> MVYSYTEKKRIRKDFGKRPQVLDVPYLLSIQLDSFQKFIEQDPEGQYGLEAAFRSVFPIQSYSGNSELQYVSYRLGEPVFDVQECQIRGVTYSAPLRVKLRLVIYEREAPEGTVKDIKEQEVYMGEIPLMTDNGTFVINGTERVIVSQLHRSPGVFFDSDKGKTHSSGKVLYNARIIPYRGSWLDFEFDPKDNLFVRIDRRRKLPATIILRALNYTTEQILDLFFEKVIFEIRDNKLQMELVPERLRGETASFDIEANGKVYVEKGRRITARHIRQLEKDDVKLIEVPVEYIAGKVVAKDYIDESTGELICAANMELSLDLLAKLSQSGHKRIETLFTNDLDHGPYISETLRVDPTNDRLSALVEIYRMMRPGEPPTREAAESLFENLFFSEDRYDLSAVGRMKFNRSLLREEIEGSGILSKDDIIDVMKKLIDIRNGKGEVDDIDHLGNRRIRSVGEMAENQFRVGLVRVERAVKERLSLGDLDTLMPQDMINAKPISAAVKEFFGSSQLSQFMDQNNPLSEITHKRRISALGPGGLTRERAGFEVRDVHPTHYGRVCPIETPEGPNIGLINSLSVYAQTNEYGFLETPYRKVTDGVVTDEIHYLSAIEEGNYVIAQANSNLDEEGHFVEDLVTCRSKGESSLFSRDQVDYMDVSTQQVVSVGASLIPFLEHDDANRALMGANMQRQAVPTLRADKPLVGTGMERAVAVDSGVTAVAKRGGVVQYVDASRIVIKVNEDEMYPGEAGIDIYNLTKYTRSNQNTCINQMPCVSLGEPVERGDVLADGPSTDLGELALGQNMRVAFMPWNGYNFEDSILVSERVVQEDRFTTIHIQELACVSRDTKLGPEEITADIPNVGEAALSKLDESGIVYIGAEVTGGDILVGKVTPKGETQLTPEEKLLRAIFGEKASDVKDSSLRVPNGVSGTVIDVQVFTRDGVEKDKRALEIEEMQLKQAKKDLSEELQILEAGLFSRIRAVLVAGGVEAEKLDKLPRDRWLELGLTDEEKQNQLEQLAEQYDELKHEFEKKLEAKRRKITQGDDLAPGVLKIVKVYLAVKRRIQPGDKMAGRHGNKGVISKINPIEDMPYDENGTPVDIVLNPLGVPSRMNIGQILETHLGMAAKGIGDKINAMLKQQQEVAKLREFIQRAYDLGADVRQKVDLSTFSDEEVMRLAENLRKGMPIATPVFDGAKEAEIKELLKLGDLPTSGQIRLYDGRTGEQFERPVTVGYMYMLKLNHLVDDKMHARSTGSYSLVTQQPLGGKAQFGGQRFGEMEVWALEAYGAAYTLQEMLTVKSDDVNGRTKMYKNIVDGNHQMEPGMPESFNVLLKEIRSLGINIELEDE;> MKDLLKFLKAQTKTEEFDAIKIALASPDMIRSWSFGEVKKPETINYRTFKPERDGLFCARIFGPVKDYECLCGKYKRLKHRGVICEKCGVEVTQTKVRRERMGHIELASPTAHIWFLKSLPSRIGLLLDMPLRDIERVLYFESYVVIEGGMTNLERQQILTEEQYLDALEEFGDEFDAKMGAEAIQALLKSMDLEQECEQLREELNETNSETKRKKLTKRIKLLEAFVQSGNKPEWMILTVLPVLPPDLRPLVPLDGGRFATSDLNDLYRRVINRNNRLKRLLDLAAPDIIVRNEKRMLQEAVDALLDNGRRGRAITGSNKRPLKSLADMIKGKQGRFRQNLLGKRVDYSGRSVITVGPYLRLHQCGLPKKMALELFKPFIYGKLELRGLATTIKAAKKMVEREEAVVWDILDEVIREHPVLLNRAPTLHRLGIQAFEPVLIEGKAIQLHPLVCAAYNADFDGDQMAVHVPLTLEAQLEARALMMSTNNILSPANGEPIIVPSQDVVLGLYYMTRDCVNAKGEGMVLTGPKEAERLYRSGLASLHARVKVRITEYEKDANGELVAKTSLKDTTVGRAILWMIVPKGLPYSIVNQALGKKAISKMLNTCYRILGLKPTVIFADQIMYTGFAYAARSGASVGIDDMVIPEKKHEIISEAEAEVAEIQEQFQSGLVTAGERYNKVIDIWAAANDRVSKAMMDNLQTETVINRDGQEEKQVSFNSIYMMADSGARGSAAQIRQLAGMRGLMAKPDGSIIETPITANFREGLNVLQYFISTHGARKGLADTALKTANSGYLTRRLVDVAQDLVVTEDDCGTHEGIMMTPVIEGGDVKEPLRDRVLGRVTAEDVLKPGTADILVPRNTLLHEQWCDLLEENSVDAVKVRSVVSCDTDFGVCAHCYGRDLARGHIINKGEAIGVIAAQSIGEPGTQLTMRTFHIGGAASRAAAESSIQVKNKGSIKLSNVKSVVNSSGKLVITSRNTELKLIDEFGRTKESYKVPYGAVLAKGDGEQVAGGETVANWDPHTMPVITEVSGFVRFTDMIDGQTITRQTDELTGLSSLVVLDSAERTAGGKDLRPALKIVDAQGNDVLIPGTDMPAQYFLPGKAIVQLEDGVQISSGDTLARIPQESGGTKDITGGLPRVADLFEARRPKEPAILAEISGIVSFGKETKGKRRLVITPVDGSDPYEEMIPKWRQLNVFEGERVERGDVISDGPEAPHDILRLRGVHAVTRYIVNEVQDVYRLQGVKINDKHIEVIVRQMLRKATIVNAGSSDFLEGEQVEYSRVKIANRELEANGKVGATYSRDLLGITKASLATESFISAASFQETTRVLTEAAVAGKRDELRGLKENVIVGRLIPAGTGYAYHQDRMRRRAAGEAPAAPQVTAEDASASLAELLNAGLGGSDNE;>MQGSVTEFLKPRLVDIEQVSSTHAKVTLEPLERGFGHTLGNALRRILLSSMPGCAVTEVEIDGVLHEYSTKEGVQEDILEILLNLKGLAVRVQGKDEV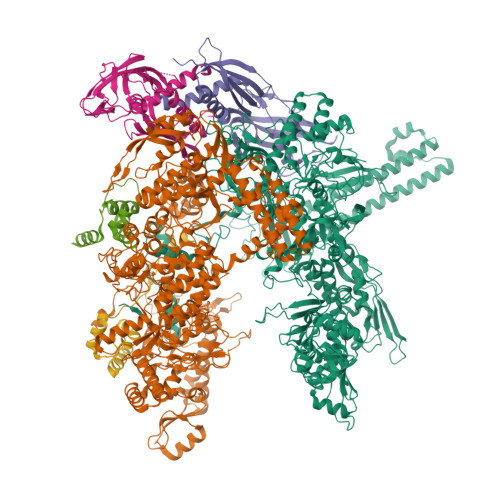ILTLNKSGIGPVTAADITHDGDVEIVKPQHVICHLTDENASISMRIKVQRGRGYVPASTRIHSEEDERPIGRLLVDACYSPVERIAYNVEAARVEQRTDLDKLVIEMETNGTIDPEEAIRRAATILAEQLEAFVDLRDVRQPEVKEEKPEFDPILLRPVDDLELTVRSANCLKAEAIHYIGDLVQRTEVELLKTPNLGKKSLTEIKDVLASRGLSLGMRLENWPPASIADE[2x];> MARVTVQDAVEKIGNRFDLVLVAARRARQMQVGGKDPLVPEENDKTTVIALREIEEGLINNQILDVRERQEQQEQEAAELQAVTAIAEGRR;> MDMFSLEDLVQNGMMEQKEPLIVGSRKELRKLCEEWGITNQRMIGNQFSAIVTFLKRGDKYSMECVERIITEAQQDKGVTYL5-[(1E,3R)-2-(2-methoxyphenyl)-3-methylpent-1-en-1-yl]furo[2,3-d]pyrimidine-2,4-diamine 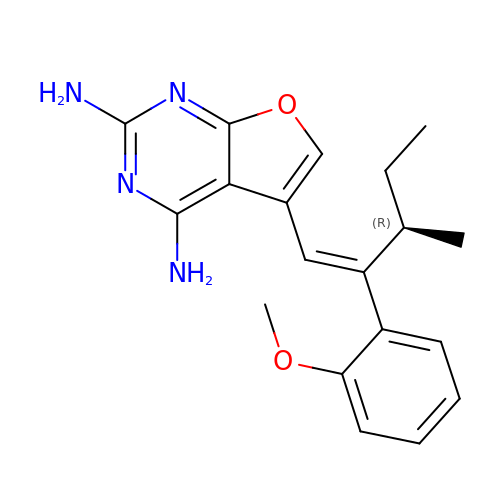| C19 H22 N4 O2 | GGNUJBNONVTLHE-ZECSTPGPSA-N In Gram-positive bacteria, nitrogen homeostasis is controlled by an operon encoding glutamine synthetase (GS), a dodecameric machine that assimilates ammonium into glutamine, and the GlnR repressor. GlnR detects nitrogen excess indirectly by binding glutamine-feedback-inhibited-GS (FBI-GS), which activates its transcription-repression function. GS generates glutamine from glutamate, ATP, and ammonium by a mechanism that involves the initial phosphorylation of the γ-carboxyl group of glutamate by ATP and the subsequent incorporation of ammonium. The structures show FBI-GS binds the GlnR C-terminal domain within its active-site cavity, juxtaposing two GlnR monomers to form a DNA-binding-competent GlnR dimer.

To visualize the active, transition state (TS) conformations of the GS proteins we reacted them with l-methionine-S-sulfoximine (MSO) in the presence of ATP and solved the structures. In these structures, the Met-Sox-P methyl group occupies the ammonium substrate binding site, thus mimicking the GS transition state and preventing further reaction. Structures of the Pp, Lm, and Sa GS-Met-Sox-P-ADP complexes were obtained to 1.98, 3.50, and 2.95 Å resolution, respectively. These structures were all dodecameric and densities for Met-Sox-P and ADP were clearly observed in each enzyme. The GS TS structures all display the same contacts to the Met-Sox-P and ADP. Strikingly, while the TS structures are similar to each other, they show significant differences, both global and local, when compared to the corresponding apo and FBI-GS-GlnR bound states (as apo and FBI-GS-GlnR conformations are the same, the state will be referred to as apo/FBI-GS-GlnR). The largest local structural changes between the GS TS and apo GS/FBI-GS-GlnR-bound states are within the active site loop regions (rmsd of apo GS/FBI-GS-GlnR versus Met-Sox-bound GS subunits is 2.0–2.5 Å for 400 corresponding Cα atoms), but the rmsds are 0.8 Å when the active site loops are not included. Moreover, superimposition of the TS dodecamer onto the apo GS or FBI-GS-GlnR bound oligomers (comparing Cα atoms of the dodecamers) results in rmsds of >3.0 Å, indicating that the catalytically induced structural changes are transmitted between subunits, causing significant alterations in the oligomeric structure. In the TS state, Asp62´ and Arg316 are repositioned to provide an optimal active site architecture. Thus, our structural analyses indicate that GS enzymes from low G + C Gram-positive bacteria adopt two distinct states, the active, TS conformation (herein termed the “A” state) and the conformation adopted by apo GS/FBI-GS-GlnR, termed the “I” or inhibited state.

>[6x]GSHMPKRTFTKEDIRKFVEEENVRYLRLQFTDILGTIKNVEVPVSQLEKVLDNEMMFDGSSIEGFVRIEESDMYLHPDLDTWVIFPWTAGQGKVARLICDVYKTDGTPFEGDPRANLKRVLKEMEDLGFTDFNLGPEPEFFLFKLDEKGEPTLELNDDGGYFDLAPTDLGENCRRDIVLELEDMGFDIEASHHEVAPGQHEIDFKYADAVTACDNIQTFKLVVKTIARKHNLHATFMPKPLFGVNGSGMHFNVSLFKGKENAFFDPNTEMGLTETAYQFTAGVLKNARGFTAVCNPLVNSYKRLVPGYEAPCYIAWSGKNRSPLIRVPSSRGLSTRIEVRSVDPAANPYMALAAILEAGLDGIKNKLKVPEPVNQNIYEMNREEREAVGIQDLPSTLYTALKAMRENEVIKKALGNHIYNQFINSKSIEWDYYRTQVSEWERDQYMKQY>GSGSMISIFIAEDQQMLLGALGSLLNLEDDMEVVGKGTTGQDAVDFVKKRQPDVCIMDIEMPGKTGLEAAEELKDTGCKIIILTTFARPGYFQRAIKAGVKGYLLKDSPSEELANAIRSVMNGKRIYAPELMEDLYSEANPLTDREKEVLELVADGKNTKEIAQELSIKSGTVRNYISMILE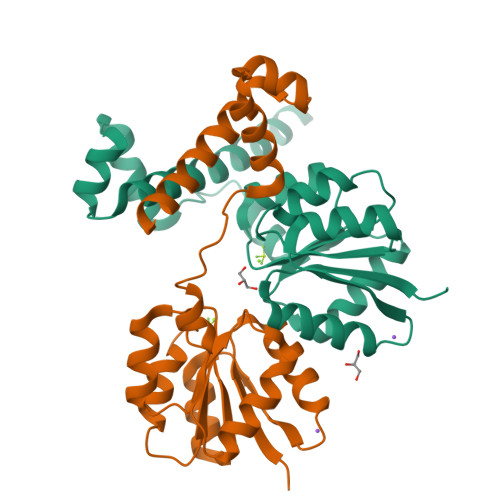KLEVKNRIEAITRSKEKGWFK[2x]Enteroviruses (EVs) comprise a large genus of positive sense RNA viruses of the family Picornaviridae and are jointly responsible for a range of serious diseases of both domestic livestock and humans. EV virions are non-enveloped ~30 nm icosahedral particles assembled from pentameric subunits comprising three structural proteins, VP0, VP1, VP3, surrounding the ~7.5 kb genome. In enteroviruses (EVs), cleavage of the structural protein VP0 into VP4 and VP2 is initiated by the incorporation of RNA into the assembling virion and is essential for infectivity. The resulting structural proteins VP0, VP3 and VP1 assemble into protomers, five of these assemble into pentamers, twelve of which assemble into icosahedral particles in the presence of a nascent VPg-coupled genome. These transient intermediate particles have been termed provirions, comprising the full complement of structural proteins encapsidating the RNA genome.

High-resolution structures of the E096A mutant EC and provirion were generated from the same dataset, exploiting the capacity of cryoEM to separate different particles within a mixed population. Initial maps showed one class containing 2739 particles (~31%) which were likely to be native conformation ECs, with no evidence of internal density corresponding to genome. After several cycles of refinement (3D auto-refinement, post processing, CTF refinement, and Bayesian polishing) the native ECs were resolved to 2.5 Å and the genome-containing provirion resolved to 2.7 Å using the gold-standard FSC (0.143). Similar to the PV native EC structure, the VP0 cleavage boundary was modelled to the same position, where the boundary interacts with a well conserved, and putatively catalytic histidine residue at the N-terminal end of the VP2 F-strand. Along with this conserved localisation, we also observed the same unusual φ and ψ angles around this site, with the carbonyl oxygens of the P1 and P1’ residues roughly facing the same direction, toward the VP2/VP3 intra-protomer interface. Unlike the PV and HRVC native EC structures, which resolved 13 and 8 residues at the N-terminal end of the scissile boundary, respectively, the E096A EC model was resolved for 5 residues upstream of the scissile site. However, while both PV and HRVC models showed discontinuous density leading to the VP0 A1 β-sheet, our native EC map allowed all residues between the scissile site and the VP0 A1 β-sheet to be modelled. After final refinements were performed, the native EC and provirion models were compared and yielded an rmsd value of 0.220 Å, suggesting that there was minimal conformational change induced by genome packaging in the presence of the E096A mutation.

> MGSQVSTQRSGSHENSNSATEGSTINYTTINYYKDSYAATAGKQSLKQDPDKFANPVKDVFTEMAAPLKSPSAEACGYSDRVAQLTIGNSTITTQAAANIIVGYGEWPSYCSDDDATAVDKPTRPDVSVNRFYTLDTKLWEKSSKGWYWKFPDVLTETGVFGQNAQFHYLYRSGFCIHVQCNASKFHQGALLVAILPEYVIGTVAGGTGTEDSHPPYIQTQPGADGFELQHPYVLDAGIPISQLTVCPHQWINLRTNNCATIIVPYMNTLPFDSALNHCNFGLLVVPISPLDFDQGATPVIPITITLAPMCSEFAGLRQAVTQ;> GFPTELKPGTNQFLTTDDGVSAPILPNFHPTPCIHIPGEVRNLLELCQVETILEVNNVPTNATSLMERLRFPVSAQAGKGELCAVFRADPGRDGPWQSTMLGQLCGYYTQWSGSLEVTFMFTGSFMATGKMLIAYTPPGGPLPKDRATAMLGTHVIWDFGLQSSVTLVIPWISNTHYRAHARDGVFDYYTTGLVSIWYQTNYVVPIGAPNTAYIIALAAAQKNFTMKLCKDTSHILQTASIQ;> GDRVADMIESSIGNSVSRALTQALPAPTGQNTQVSSHRLDTGEVPALQAAEIGASSNTSDESMIETRCVLNSHSTAETTLDSFFSRAGLVGEIDLPLEGTTNPNGYANWDIDITGYAQMRRKVELFTYMRFDAEFTFVACTPTGQVVPQLLQYMFVPPGAPKPESRESLAWQTATNPSVFVKLTDPPAQVSVPFMSPASAYQWFYDGYPTFGEHKQEKDLEYGACPNNMMGTFSVRTVGSSKSKYALVVRIYMRMKHVRAWIPRPMRNQNYLFKANPNYAGDSIKPTGTSRNAITTL> KPEPTDEEWELIKTVTEAHVATNAQGSHWKQKRKFLPEDIGQAPIVNAPEGGKVDLEAFSHFTKIITPAITRVVDFAKKLPMFCELPCEDQIILLKGCCMEIMSLRAAVRYDPESETLTLNGEMAVTRGQLKNGGLGVVSDAI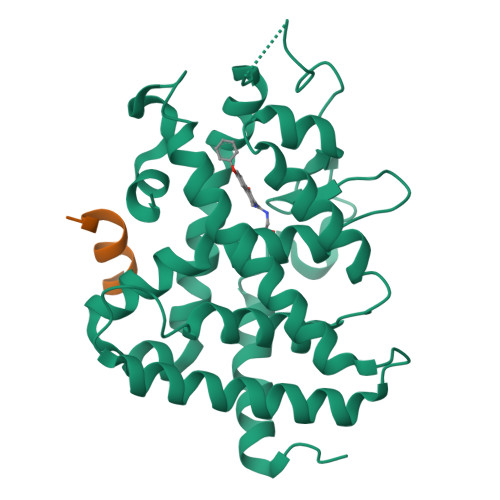FDLGMSLSSFNLDDTEVALLQAVLLMSSDRPGLACVERIEKYQDSFLLAFEHYINYRKHHVTHFWPKLLMKVTDLRMIGACLASRFLHMKVECPTELFPPLFLEVF;> ENALLRYLLDK>SMSNANPFFSQSLAERDASVRGAILKELERQQSQVELIASENIVSRAVLDAQGSVLTNKYAEGYPGKRYYGGCEFADEVEALAIERVKRLFNAGHANVQPHSGAQANGAVMLALAKPGDTVLGMSLDAGGHLTHGAKPALSGKWFNALQYGVSRDTMLIDYDQVEALAQQHKPSLIIAGFSAYPRKLDFARFRA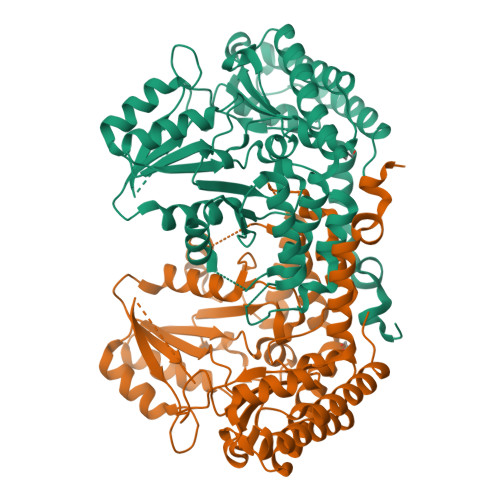IADSVGAKLMVDMAHIAGVIAAGRHANPVEHAHVVTSTTHKTLRGPRGGFVLTNDEEIAKKINSAVFPGLQGGPLMHVIAGKAVAFGEALTDDFKTYIDRVLANAQALGDVLKAGGVDLVTGGTDNHLLLVDLRPKGLKGAQVEQALERAGITCNKNGIPFDPEKPTITSGIRLGTPAGTTRGFGAAEFREVGRLILEVFEALRTNPEGDHATEQRVRREIFALCERFPIY[4x]>GMNISNLINADVDEKGFVSDKLRD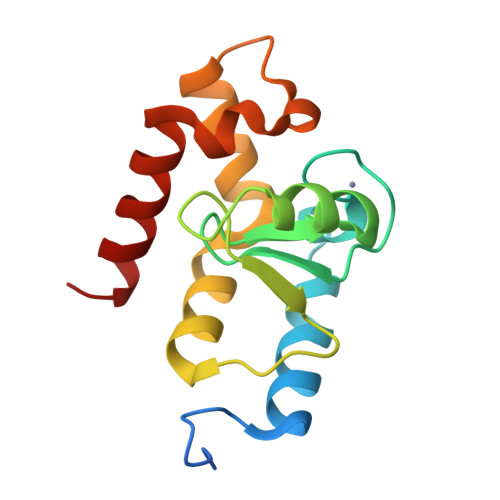NFFQIVRNRPENRTCFDCESRNPTWLSLSFAVFICLNCSSDHRKMGVHISFVRSSDLDKFTPIQLVRMDIGGNGRARNYFKQVLGVNFSPKTKEYASSICGRQYKQILDSEISE[2x]>[2x]SNAMRTFDLVTGESLFVNDLRVVRWEQYGLGTAMPFQAMWYSVPPGDESPIDQHPELELSIVVAGTAHVTVGDT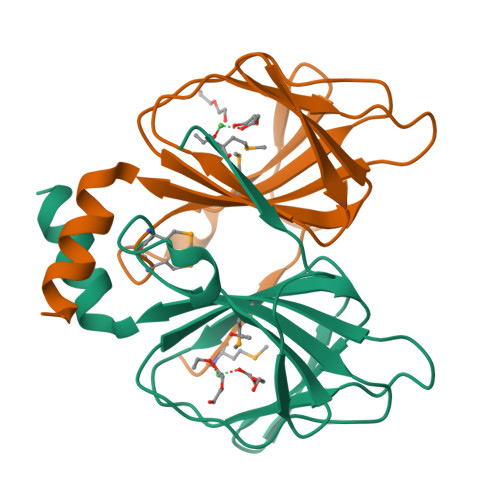VHEVPHGNAFLLNSLEAHVVQNRSADEVLTVFSAYWYPEAATAAAEALA>MADYKVKDISLAEWGRKAIELAENEMPGLMELRREYGPSQPLKGAKIAGCLHMTVQTAVLIETLKALGAELRWSSCNIFSTQDNAAAAIAKTGVPVFAWKGETDEEYEWCIAQTVKGFSGDGLPNMILDDGGDLTNLVIDRYPELVPKIFGISEETTTGVKNLYKRLSKGNLPISAINVNDSVTKSKFDNLYGCRESLVDGIKRATDVMIAGKTCCVCGYGDVGKGCAAALRAFGARVVVTEVDPINALQASMEGYQVALVEDVMADAHIFVTTTGNDDIITSDHFPHMRDDAIVCNIGHFDTEIQVGWLEANAKEHVEIKPQVDRYTMENGRHIILLAKGRLVNLGCASGHPSFVMSNSFTNQVLAQIELWSNRDNGKYPRGDKAGVFFLPKALDEKVAALHLAHVGAKLTKLTPKQAEYINCPVNGP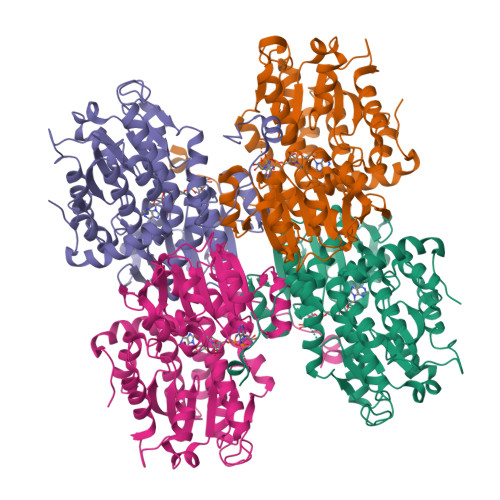FKPDHYRY[4x]> XTTLSDKDKSTVKALWGKISKSADAIGADALGRMLAVYPQTKTYFSHWPDMSPGSGPVKAHGKKVMGGVALAVSKIDDLTTGLGDLSELHAFKMRVDPSNFKILSHCILVVVAKMFPKEFTPDAHVSLDKF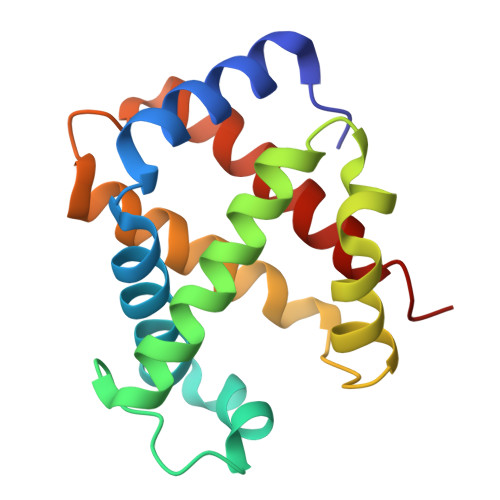LASVALALAERYR>[4x]GSHMATFPELLRPLKLGRYTLRNRIIMAPLTRCQATEDGHVPRTESMLKYYEDRASAGLIIAEATMVQPNYTGFLTEPGIYSDAQIEEWRKIVDAVHKKGGLIFLQLIHAGRAGIPEKILQQPKSDQDPLAGRLLAASAIPIKDHRIPAYFAASGEKETYGVPEELTDDEVRNGIIPLFVEGAKNAIFKAGFDGVEIHGANGYLLDAFFRESSNKRQSGPYAG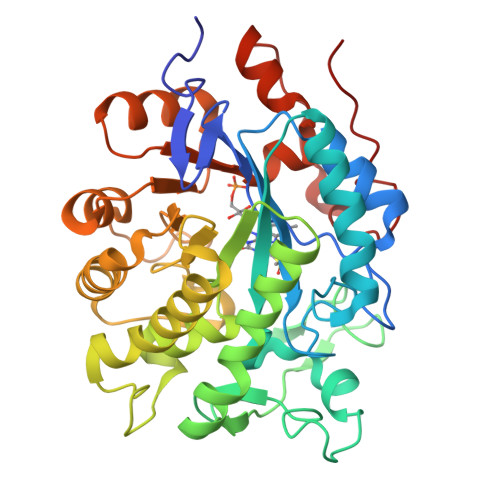TTIDTRCQLIYDVTKSVCDAVGSDRVGLRISPLNGVHGMIDSNPEALTKHLCKKIEPLSLAYLHYLRGDMVNQQIGDVVAWVRGSYSGVKISNLRYDFEEADQQIREGKVDAVAFGAKFIANPDLVERAQHDWPLNEPRPETYYTRTAVGYNDYPTYNK> VPISPIETVPVKLKPGMDGPKVKQWPLTEEKIKALVEICTEMEKEGKISKIGPENPYNTPVFAIKKKDSTKWRKLVDFRELNKRTQDFWEVQLGIPHPAGLKKKKSVTVLDVGDAYFSVPLDEDFRKYTAFTIPSINNETPGIRYQYNVLPQGWKGSPAIFQSSMTKILEPFAAQNPDIVIYQYMDDLYVGSDLEIGQHRTKIEELRQHLLRWGLTTPDKKHQKEPPFLWMGYELHPDKWTVQPIVLPEKDSWTVNDIQKLVGKLNWASQIYPGIKVRQLSKLLRGTKALTEVIPLTEEAELELAENREILKEPVHGVYYDPSKDLIAEIQKQGQGQWTYQIYQEPFKNLKTGKYARMRGAHTNDVKQLTEAVQKITTESIVIWGKTPKFKLPIQKETWETWWTEYWQATWIPEWEFVNTPPLVKLWYQLEK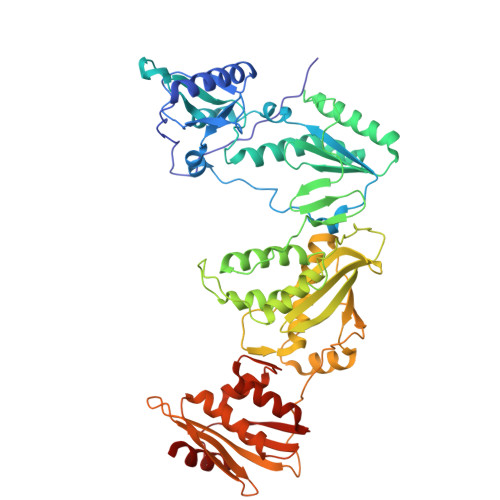EPIVGAETFYVDGAANRETKLGKAGYVTNKGRQKVVPLTNTTNQKTELQAIYLALQDSGLEVNIVTDSQYALGIIQAQPDKSESELVNQIIEQLIKKEKVYLAWVPAHKGIGGNEQVDKLVSA Spermidine/spermine N-acetyltransferases (SSATs) are catabolic enzymes that acetylate polyamines and are critical for maintaining intracellular polyamine homeostasis. SpeG is an SSAT protein found in a variety of bacteria, including the human pathogen Vibrio cholerae. This protein adopts a dodecameric structure and contains an allosteric site, making it unique compared to other SSATs. The allosteric site is located between monomers that form the hexamers of the dodecamer, and some evidence has been provided that shows when polyamine binds to these sites, the dodecamer tightens.

Our analysis of the spm-bound structure of VcSpeG showed these two regions form potentially significant contacts: π-π interactions between F32 and F149 and an H-bond between R25 and N152. To elucidate whether these residues could be important for stabilizing the interaction between these two regions of VcSpeG, we created three point mutants: N152L, F149A, and F149G (R3C4-R3C6). We substituted leucine for asparagine at position 152 to retain the overall structural similarity of the residue but remove the ability to H-bond, and we substituted alanine and glycine for phenylalanine at position 149 to potentially decrease the ability of this residue to form hydrophobic interactions. During our kinetic analyses we found the VcSpeG N152L (R3C4), F149A (R3C5), and F149G (R3C6) mutant enzymes still retained reasonably high activity toward spm. The catalytic efficiency of the N152L mutant increased slightly (1.2-fold), and the F149A and F149G mutants decreased 1.4- and 5.3-fold, respectively compared to WT. Our analysis of the spm-bound homology models for the R3C4-R3C6 constructs showed all three retained spm in the allosteric site. On the other hand, when we replaced phenylalanine with alanine (R3C5) and with glycine (R3C6) at position 149, the π-π interactions between F32 and F149 were removed and the H-bond between R25 and N152 side chains remained. While this H-bond is still possible in the R3C6 homology model, it may ultimately be disrupted due to the greater flexibility of a glycine substitution at position 149. The single point mutants we tested in Region 3 (F149, N152; R3C4-R3C6) were insufficient to totally inhibit enzyme activity. In cases where only a single residue in this region was altered (R3C4-R3C6), the disruption to the activity was far less.

>MNSQLTLRALERGDLRFIHNLNNNRNIMSYWFEEPYESFDELEELYNKHIHDNAERRFVVEDAQKNLIGLVELIEINYIHRSAEFQIIIAPEHQGKGFARTLINRALDYSFTILNLHKIYLHVAVENPKAVHLYEECGFVEEGHLVEEGFINGRYQDVKRMYILQSKYLNRSE[3x]>[4x]GASMTIEDEYSGPKLEDGKVTISFMKELMQWYKDQKKLHRKCAYQILVQVKEVLSKLSTLVETTLKETEKITVCGDTHGQFYDLLNIFELNGLPSETNPYIFNGDFVDRGS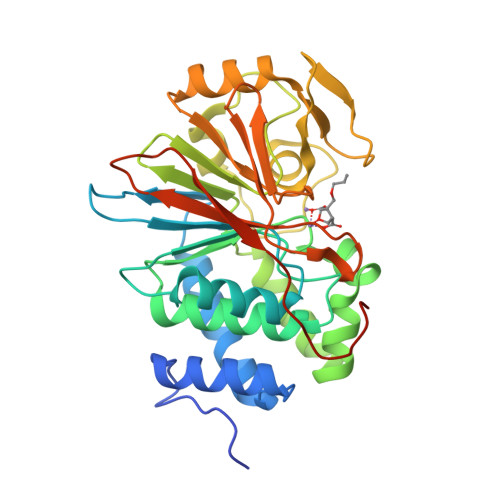FSVEVILTLFGFKLLYPDHFHLLRGNHETDNMNQIYGFEGEVKAKYTAQMYELFSEVFEWLPLAQCINGKVLIMHGGLFSEDGVTLDDIRKIERNRQPPDSGPMCDLLWSDPQPQNGRSISKRGVSCQFGPDVTKAFLEENNLDYIIRSHEVKAEGYEVAHGGRCVTVFSAPNYCDQMGNKASYIHLQGSDLRPQFHQFTAVPHPNVKPMAYANTLLQLGMM(2R)-1,1,1-trifluoropropan-2-yl {(2R,4R,6S,12Z,13aS,14aR,16aS)-2-[(7-methoxy-3-methylquinoxalin-2-yl)oxy]-14a-[(1-methylcyclopropane-1-sulfonyl)carbamoyl]-5,16-dioxo-1,2,3,5,6,7,8,9,10,11,13a,14,14a,15,16,16a-hexadecahydrocyclopropa[e]pyrrolo[1,2-a][1,4]diazacyclopentadecin-6-yl}carbamate 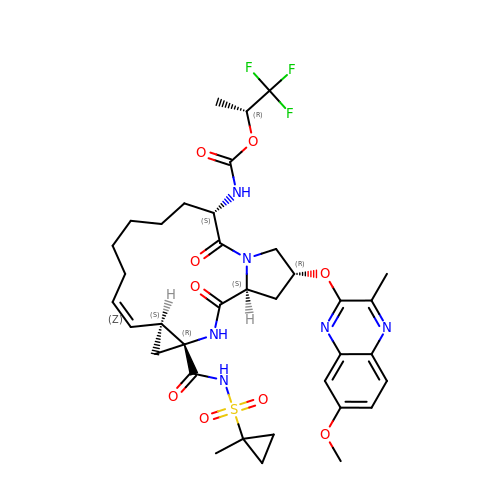| C36 H45 F3 N6 O9 S | RTCPQVJDZHADDP-XVMCOVDDSA-N> GSHMVPDTPTRLVFSALGPTSLRVSWQEPRCERPLQGYSVEYQLLNGGELHRLNIPNPAQTSVVVEDLLPNHSYVFRV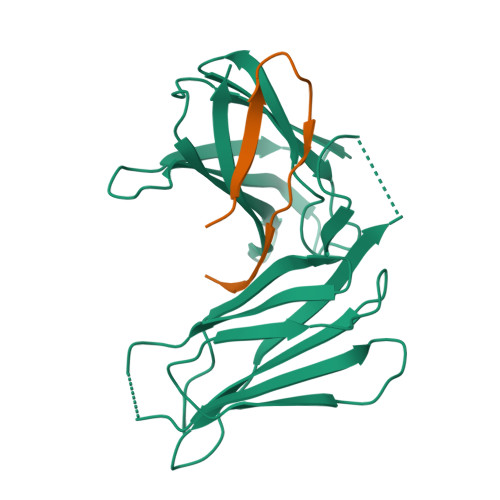RAQSQEGWGREREGVITIESQVHPQSPLCPLPGSAFTLSTPSAPGPLVFTALSPDSLQLSWERPRRPNGDIVGYLVTCEMAQGGGPATAFRVDGDSPESRLTVPGLSENVPYKFKVQARTTEGFGPEREGIITIES;> DSNENLLLVHCGPTLINSCISFGSESFDGH> GSHMIQAYLGLGSNIGDRESQLNDAIKILNEYDGISVSNISPIYETAPVGYTEQPNFLNLCVEIQT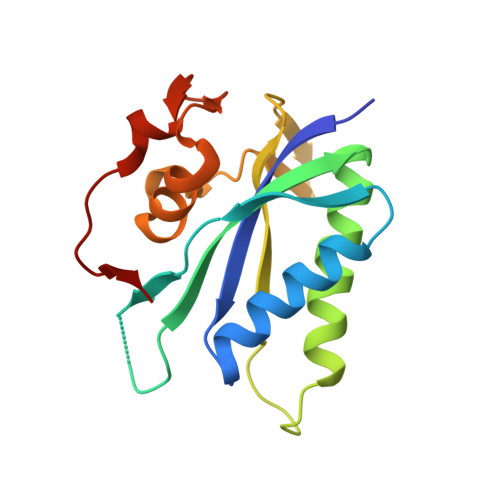TLTVLQLLECCLKTEECLHRIRKERWGPRTLDVDILLYGEEMIDLPKLSVPHPRMNERAFVLIPLNDIAANVVEPRSKLKVKDLVFVNDSVKRYK>[2x]DVSFSLSGSSSTSYSKFIGALRKALPSNGTVYNITL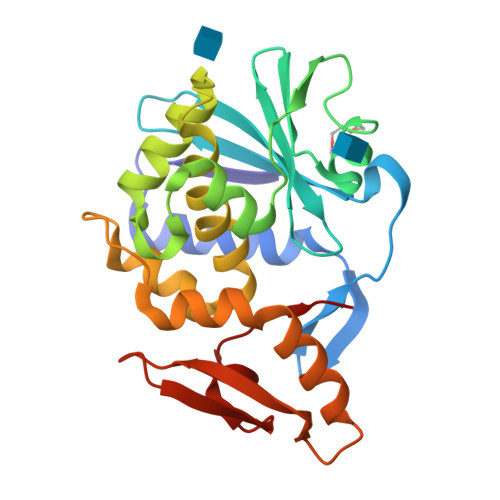LLSSASGASRYTLMKLSNYDGKAITVAIDVTNVYIMGYLVNSTSYFFNESDAKLASQYVFAGSTIVTLPYSGNYEKLQTAAGKIREKIPLGFPALDSAITTLFHYDSTAAAAAFLVIIQTTAESSRFKYIEGQIIMRISKNGVPSLATISLENEWSALSKQIQLAQTNNGTFKTPVVIMDAGGQRVEIGNVGSKVVTKNIQLLLN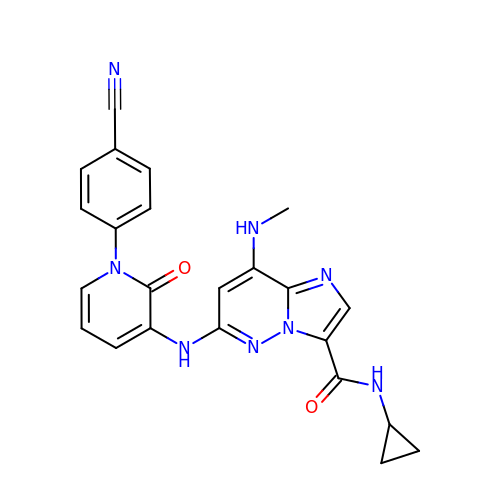6-{[1-(4-cyanophenyl)-2-oxo-1,2-dihydropyridin-3-yl]amino}-N-cyclopropyl-8-(methylamino)imidazo[1,2-b]pyridazine-3-carboxamide | C23 H20 N8 O2 | LMOIQLXOGZDGRD-UHFFFAOYSA-N>[3x]EFPRNCKDLLDRGYFLSGWHTIYLPDCRPLTVLCDMDT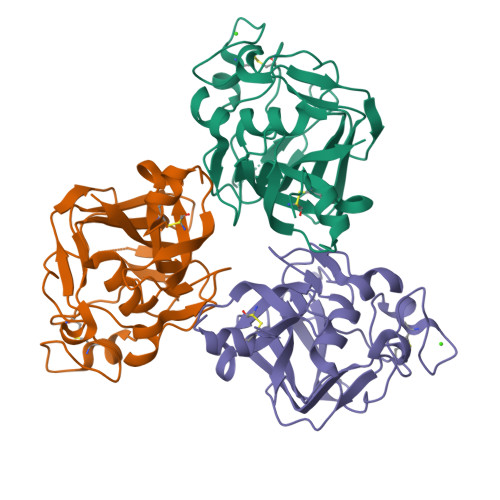DGGGWTVFQRRMDGSVDFYRDWAAYKQGFGSQLGEFWLGNDNIHALTAQGSSELRVDLVDFEGNHQFAKYKSFKVADEAEKYKLVLGAFVGGSAGNSLTGHNNNFFSTKDQDNDVSSSNCAEKFQGAWWYADCHASNLNGLYLMGPHESYANGINWSAAKGYKYSYKVSEMKVRPAFLEQKLISEEDLNSAVDHHHHHH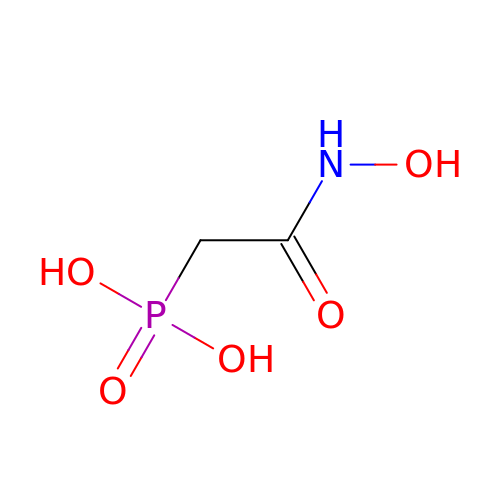PHOSPHONOACETOHYDROXAMIC ACID | C2 H6 N O5 P | LDKRAXXVBWHMRH-UHFFFAOYSA-N> MGKYLLPTAAAGLLLLAAQPAMDFTIQDIRVEGLQRTEPSTVFNYLPVKVGDTYNDTHGSAIIKSLYATGFFDDVRVETADGQLLLTVIERPTIGSLNITGAKMLQNDAIKKNLESFGLAQSQYFNQATLNQAVAGLKEEYLGRGKLNIQITPKVTKLARNRVDIDITIDEGKSAKITDIEFEGNQVYSDRKLMRQMSLTEGGIWTWLTRSDRFDRQKFAQDMEKVTDFYQNNGYFDFRILDTDIQTNEDKTRQTIKITVHEGGRFRWGKVSIEGDTNEVPKAELEKLLTMKPGKWYERQQMTAVLGEIQNRMGSAGYAYSEISVQPLPNAGTKTVDFVLHIEPGRKIYVNEIHITGNNKTRDEVVRRELRQMESAPYDTSKLQRSKERVELLGYFDNVQFDAVPLAGTPDKVDLNMSLTERSTGSLDLSAGWVQDTGLVMSAGVSQDNLFGTGKSAALRASRSKTTLNGSLSFTDPYFTADGVSLGYDIYGKAFDPRKASTSVKQYKTTTAGGGVRMGIPVTEYDRVNFGLAAEHLTVNTYNKAPKRYADFIRKYGKTDGADGSFKGLLYKGTVGWGRNKTDSASWPTRGYLTGVNAEIALPGSKLQYYSATHNQTWFFPLSKTFTLMLGGEVGIAGGYGRTKEIPFFENFYGGGLGSVRGYESGTLGPKVYDEYGEKISYGGNKKANVSAELLFPMPGAKDARTVRLSLFADAGSVWDGRTYTAAENGNNKSVYSENAHKSTFTNELRYSAGGAVTWLSPLGPMKFSYAYPLKKKPEDEIQRFQFQLGTTF;> MGKYLLPTAAAGLLLLAAQPAMATQGTADKDAQITQDWSVEKLYAEAQDELNSSNYTRAVKLYEILESRFPTSRHARQSQLDTAYAYYKDDEKDKALAAIERFRRLHPQHPNMDYALYLRGLVLFNEDQSFLNKLASQDWSDRDPKANREAYQAFAELVQRFPNSKYAADATARMVKLVDALGGNEMSVARYYMKRGAYIAAANRAKKIIGSYQNTRYVEESLAILELAYKKLDKPQLAADTRRVLETNFPKSPFLTHAWQPDDMPWWRYWH;> MQLRKLLLPGLLSVTLLSGCAMDSVE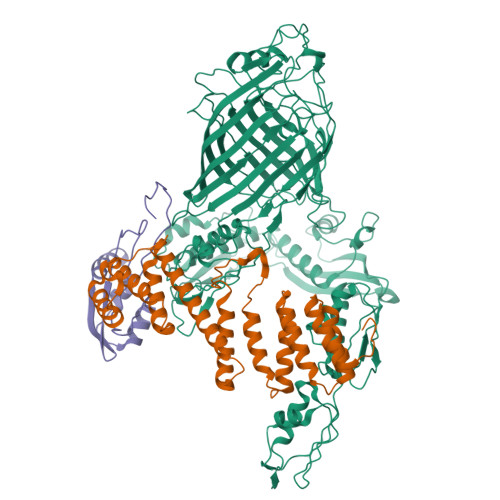RVSLFPSYKLKIIQGNELEPRAVAALRPGMTKDQVLLLLGSPILRDAFHTDRWDYTFNTSRNGIIKERSNLTVYFENGVLVRTEGDALQNAAEALRAKQNADKQHHHHHHHHHH> GAMETRLNVVLRGIAFGARPGAVIEEGGKQQVYLQGERLDSHNAVIEEINRDHVMLRYQGKIERLSLA;> GAMAEEATFTANFKDTDLKSFIETVGANLNKTIIMGPGVQGKVSIRTMTPLNERQYYQLFLNLLEAQGYAVVPMYIDTNNDGYIEGDELVLKVVKSSA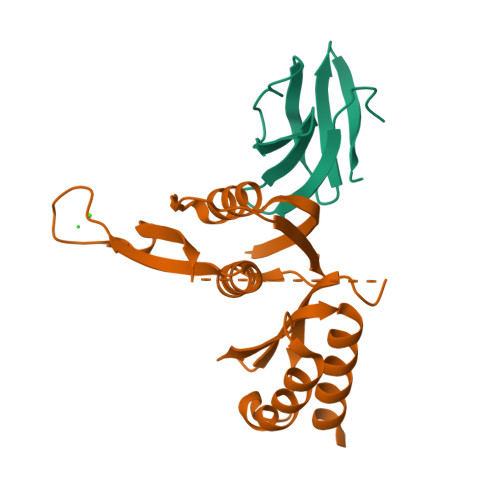AKVEPLPLVGEGSDNYAGDEMVTKVVPVRNVSVRELAPILRQMIDSAGSGNVVNYDPSNVIMLTGRASVVERLTEVIQRVDHA>[2x]MASHHHHHHHHHHENLYFQGSKRHIPVVTDIYSVEDHRLEDTTHLQYAPNAIKTEGKGSGSGPAVCKKVTEHERCTTSIMDKLTAFFGVMPRGTTPRAPVRFPTSLLKIRRGLETGWAYTHQGGISSVDHVTCGKDLLVCDTMGRTRVVCQSNNKMTDESEYGVKTDSGCPEGARCYVFNPEAVNISGTKGAMVHLQKTGGEFTCVTASGTPAFFDLKNLKGWAGLPIFEASSGRVVGRVKVGKNEDSKPTKLMSGIQTVSKSATDLTEMVKKITTMNRGEFRQITLATGAGKTTELPRSVIEEIGRHKRVLVLIPLRAAAESVYQYMRQKHPSIAFNLRIGEMKEGDMATGITYASYGYFCQMSQPKLRAAMVEYSFIFLDEYHCATPEQLAIMGKIHRFSENLRVVAMTATPAGTVTTTGQKHPI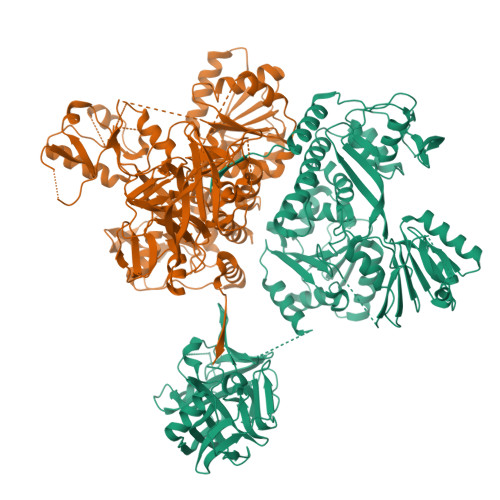EEFIAPEVMKGEDLGSEYLDIAGLKIPVEEMKNNMLVFVPTRNMAVEAAKKLKAKGYNSGYYYSGEDPSNLRVVTSQSPYVVVATNAIESGVTLPDLDVVVDTGLKCEKRIRLSPKMPFIVTGLKRMAVTIGEQAQRRGRVGRVKPGRYYRSQETPVGSKDYHYDLLQAQRYGIEDGINITKSFREMNYDWSLYEEDSLMITQLEILNNLLISEELPMAVKNIMARTDHPEPIQLAYNSYETQVPVLFPKIRNGEVTDTYDNYTFLNARKLGDDVPPYVYATEDEDLAVELLGLDWPDPGNQGTVEAGRALKQVVGLSTAENALL>[8x]SLSLGDQKPATIYAPTVRVTPNPAWPQVSWQLLVAKPSAARIIDSPRINVRPTPGELQVYHGAGWAQPATDMLEDSVVRAFEDSGKIAAVARIGA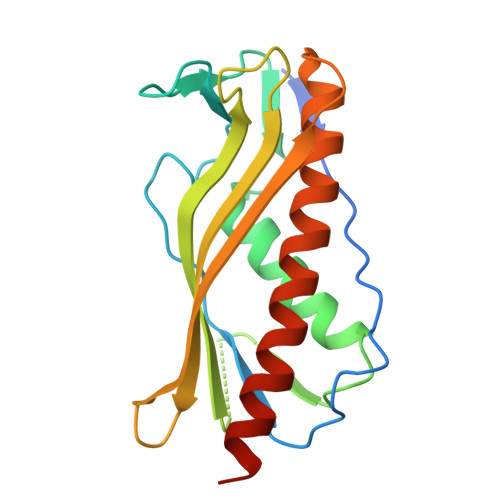GIRSDYKLAIDVRRFESDYAGQSLPAATIELNAKLLHSSDQRVVASRTFTVARPSSSTDTAAVAAAFEQALTQVTTELVGWTLITGQQDSQTLPRAL>SVYSNSPVPVYKDLNAVGPLSELTISPHASVEVFRIDTPIIPESRKSLRVVNTGLANSVTAKFYWSHSFTSEWFESGSIDVGLGEDKV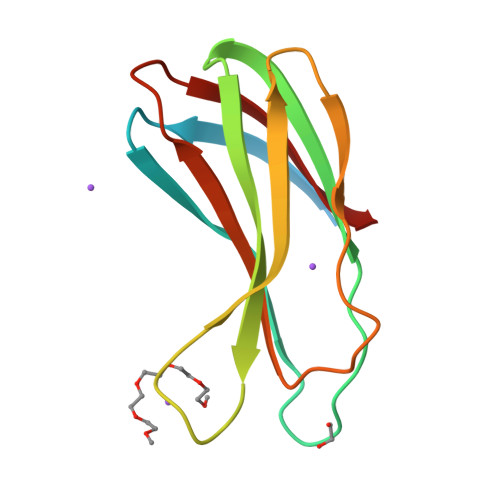LNVPSNSFYYSKFVIYNNTDKVAYVTANLV[4x]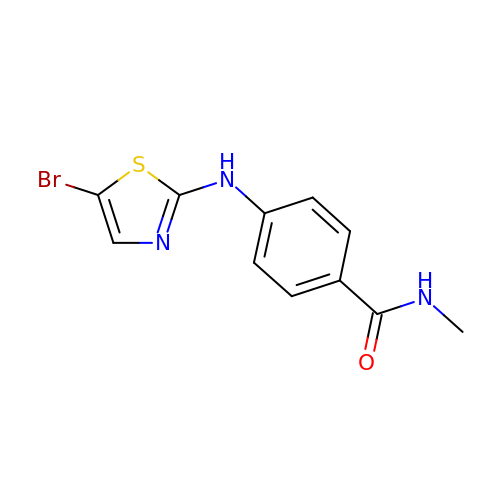4-[(5-bromo-1,3-thiazol-2-yl)amino]-N-methylbenzamide | C11 H10 Br N3 O S | IMMYNZJEOGNQTM-UHFFFAOYSA-N> MASYAELF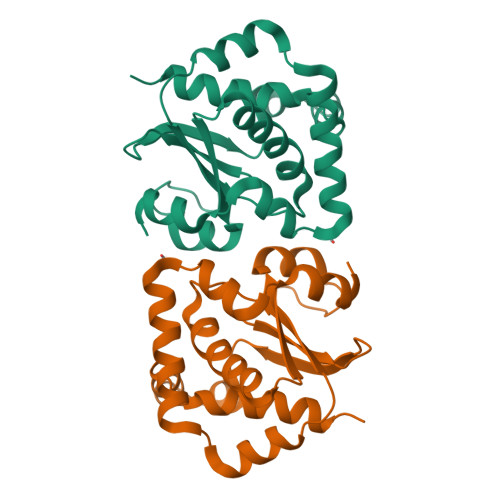DIGEDFAAFVGHGLATEQGAVARFRQKLESNGLPSALTERLQRIERRYRLLVAGEMWCPDCQINLAALDFAQRLQPNIELAIISKGRAEDDLRQRLALERIAIPLVLVLDEEFNLLGRFVERPQAVLDGGWFDITAYLWGGHLEHAIGDVLAIIEGAAHHHHHH>GSHMTDHDERTFVMVKPDGVQRGLIGDIVTRLE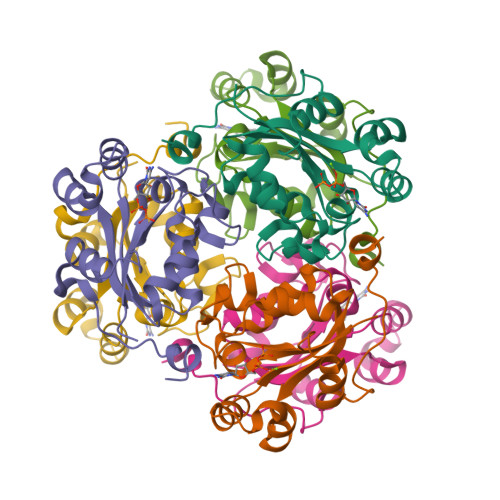TKGLKMVGGKFMRIDEELAHEHYAEHEDKPFFDGLVSFITSGPVFAMVWEGADATRQVRQLMGATDAQDAAPGTIRGDYGNDLGHNLIHGSDHEDEGANEREIALFFDDDELVDWDRDASAWVYEDLADHD[9x]> GAMARCERLRGAALRDVLGRAQGVLFDCDGVLWNGERAVPGAPELLERLARAGKAALFVSNNSRRARPELALRFARLGFGGLRAEQLFSSALCAARLLRQRLPGPPDAPGAV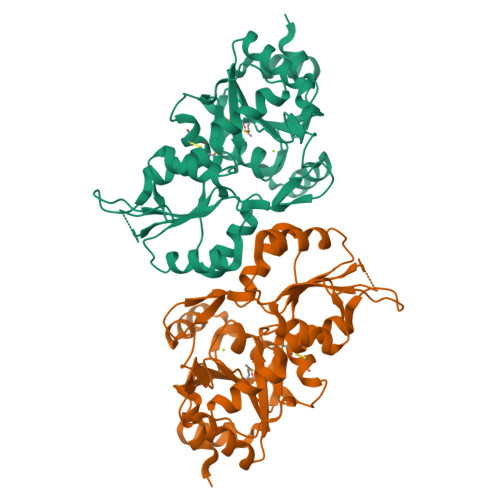FVLGGEGLRAELRAAGLRLAGDPSAGDGAAPRVRAVLVGYDEHFSFAKLREACAHLRDPECLLVATDRDPWHPLSDGSRTPGTGSLAAAVETASGRQALVVGKPSPYMFECITENFSIDPARTLMVGDRLETDILFGHRCGMTTVLTLTGVSRLEEAQAYLAAGQHDLVPHYYVESIADLTEGLED Aryl polyenes (APE) are one of the most widespread secondary metabolites among gram-negative bacteria. APE biosynthesis gene clusters harbor two ketosynthases (KSs): the heterodimeric KS-chain length factor complex, ApeO-ApeC, and the homodimeric ketoacyl-acyl carrier protein synthase I (FabB)-like KS, ApeR. To understand the structural basis of the functional redundancy in the two KSs, AbApeO-AbApeC and AbApeR, from the APE BGC of A. baumannii, we determined the crystal structures of AbApeO-AbApeC and AbApeR in the absence of substrates. Therefore, the two KSs function complementarily in the generation of APE to enhance its production.

In the crystal form, there were two heterodimers in the asymmetric units; we focused on the structure of the first heterodimer (chain A and chain B), which had a relatively lower overall temperature B-factor than that of chain C and chain D in the structure. The overall structure was superposed with the X. doucetiae KS-CLF complex with an r.m.s.d. of 0.68 Å. However, AbApeC was composed of only one thiolase fold domain. Among the conserved residues, Arg30 and Arg31 residues in AbApeC appeared to be important for the ACP-KS-CLF interactions, because ACPs are negatively charged proteins. The cavity of AbApeC-AbApeO was characterized by its asymmetric shape because of the lack of cavity belonging to AbApeC as observed in other CLFs. The cavity was lined by residues from both AbApeO and AbApeC. The volume of the cavity was 120.4 Å3, as calculated using the SiteMap tool of Maestro software package, 2020–2 release. His268 residue in AbApeR was a part of the loop sterically linked to the loop containing the gating residue Phe391 in E. coli FabB. Inside the AbApeO cavity, in addition to the gating residue Phe387, residues Phe85, Val89, Ala166, and Phe205 near the entrance of the active site cavity were strictly conserved, underlining the importance of these residues in function. AbApeO-AbApeC had a comparatively stringent Kd of 7.4 × 10−8 M (N = 1.63) for holo ACP1. However, the 6EN-AbApeO-AbApeC model indicated that the bound substrate entered the cavity, such that the full elongation of the substrate up to six conjugated double bonds was possible, as observed previously in XdApeO-XdApeC.

>MVTLHLAHLTLTHAQPSYAALECIPAMQRRRLSPLAKLALNTAISSLDGRSADYIVWVSKYGDEAKTLNILQDVLNDQTPSPTQFSTSVHNAISGLYSILCQDDTPSTSLSCSWTEGLIEAYALLKSMPEIKRVLVVAYDEPLPNIYAEAINFPAYAMAAVVTLEQPNLQITAWTHTDEAEAPAFAHFWQDADQLTSAFGWNKC[2x];>[2x]MKHLPSENAAPMAVGIQFSVGLSALGCELNQIKQALQQPQQTLSLRDDLIADRDVWVGQYTHPLCSSVPDAMRSVDSRNLRFALTALSKIETELKAYTASFENKRLAIVVGTSTSGIADNELLLKQYFQGQTDLSISHYPQEMSCLAKALQQYLGWEGPAYTISTACSSSAKALAAGQRLLHADLADVVLVGGVDTLCKLTLNGFNSLESLSAHICQPCGISRDGINIGEAAAFFVLSKEQAPVMLMGAGETMDAWHISAPHPEGKGAALAMQRALDMAHISAQEVGYINLHGTATPQNDAMEIKAVRQVFGVYQVALSSTKHKTGHCLGAAGAIEAFICEQVLKDQSWLPLHQNVEIDPDLVDQNYVQEAELTQPIRYVMSNSFAFGGSNISLVFGVKP> MDGSRGTAPGGDDLRGDRRDSYQGEDREDSHLLGALEDGNHQQSQGHGGGSGFYHHNVNSSSASVLEGVEMAHDELFAGPVAESVPTSVSAFSHRHGRAESVASFSFYHEQDDQREELEAPPGSLGARLSIDDLDELPFEEEGLSESEMPEQLDTFGIDLEWGSMNNGYPLIRRSSTHSQFSAHHRLLRRESGVSAASGYTGGRSSQKMRLDNDDLTIAISGFITNRIGFAIYIVLCVLTGGIAWLFLRWYPKYYVKLVGCATPFRDCQWVVIEDHFNKMTILSIRVKPYNRPLSTVFGTPSRATSWPLAQDPDPVLRELRSITYCYYKFYYHPVLDKFFCCNGWKDPQWNSMQNARSGLHGDEKAHREAVFGPNSIDVDEQSILQLLVSEILTPFYAFQVFSLILWLCDEYYYYAAAILLISAGSIITSLL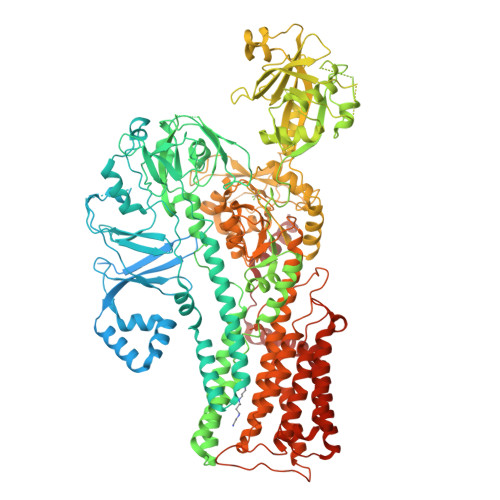ETKETRRRLREMSRFECEVRVFRGGFWRTFPSSDLVPGDVYEVSDPSLTQIPADSLLLTGDCIVNESMLTGESVAVSKTPATNETLAKLNPAASTFSHDVDKHFLYCGTKLIRARQRLADTDEAAAVALVVRTGFNTTRGALVRSMLVPKPSKFKFYEDSFRYLKVMGCLAGLAFIVSLVNFIRLKLHWTLILLRALDLLTIVVPPALPATLTIGTSFAVQRLKGKKIFCTSPQRVNVGGKIDLMCFDKTGTLTEEGLDVLGIRVASRVSNRFTELLTNVDDLTWSCDSVSNGDEVKPADHVDGSSLKKDKTKPLDPYRAALYVMASCHSLRIVDGVAVGDPLEVKMFEFTGWSYEEGFIAGEVISTEGRGDISPSIARPPRYMTSQEMSIGEAPPAVGVLRAFDFNPLLRRSSVIARVVGNSGGYALVKGSPECMPEICRPETLPSDFDELLSYYTHAGYRVIACATKRIPKLNLVSVNRMTRDEVESGLDFVGFIIFENKLKPTTTSVIKELLSSNIGTVMITGDNIRTAVSVARQCGIIEEHAHCYMPRFIEGNADDCNAKLRWESINNPALELDPWTLLPMPVPPQTDASLPYDVSNIRNYAIAVTGDVFRWIVDHAPTDVLHRMLVLGKVYARMSPDEKQELVKKFQSIDYSCGFCGDGANDCAALKAADVGISLSEAEASVAAPFTSQIFDIRCVPEVIREGRASLVTSFSCFKYMSLYSFIQFTSVSFLYVSASNLGDFQFLYIDLMLILPIAVFMSWAGPHSKLCAKRPVSDLVSRKVLVPLLSHVFVCVMIQALAWVAVRQQPWYIPPIVDTEKSNIENSENTTLFFASCFEYILSGVVLNAGRPFRQSPLETWPFLSAVAVTLIATLLMLLVPPYWLFEFMQLTWMSWTFKITLIAFGFVYFLIAWTGEHYLFLWLARFLGRMRQRLFKQPKQRKLYKIVKEKLVFENLYF>[6x]GSMLELPPVASLKGKSITSAEQFSRADIYALIHLASAMQRKIDAGEVLNLLQGRIMTPLFFEDSSRTFSSFCAAMIRLGGSVVNFKVEASSINKGETLADTIRTLDSYSDVLVMRHPRQDAIEEALSVAQHPILNAGNGAGEHPTQALLDTLTIHSELGSVDGITIALIGDLKMGRTVHSLLKLLVRNFSIKCVFLVAPDALQMPQDV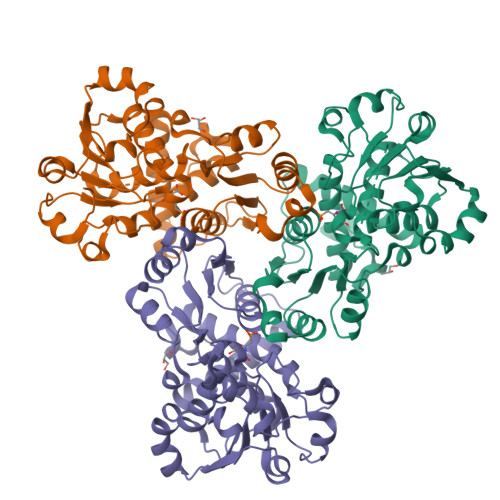LEPLQHEIATKGVIIHRTHALTDEVMQKSDVLYTTRLQKERFMASTSDDAAALQSFAAKADITIDAARMRLAKEKMIVMHPLPRNDELSTTVDADPRAAYFRQMRYGMFMRMAILWSVLA> MVSLPRMVYPQSKVLTPCRKDVL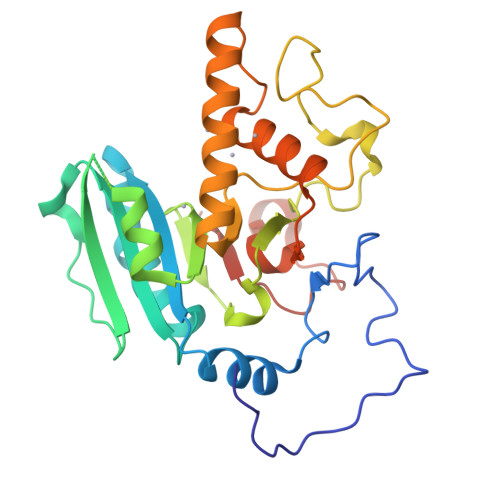VVTPWLAPIVWEGTFNIDILNEQFRLQNTTIGLTVFAIKKYVAFLKLFLETAEKHFMVGHRVHYYVFTDQPAAVPRVTLGTGRQLSVLEVRAYKRWQDVSMRRMEMISDFCERRFLSEVDYLVCVDVDMEFRDHVGVEILTPLFGTLHPGFYGSSREAFTYERRPQSQAYIPKDEGDFYYLGRFFGGSVQEVQRLTRACHQAMMVDQANGIEAVWHDESHLNKYLLRHKPTKVLSPEYLWDQQLLGWPAVLRKLRFTAVPKNHQAVRNP> MGSDKIHHHHHHLPKLR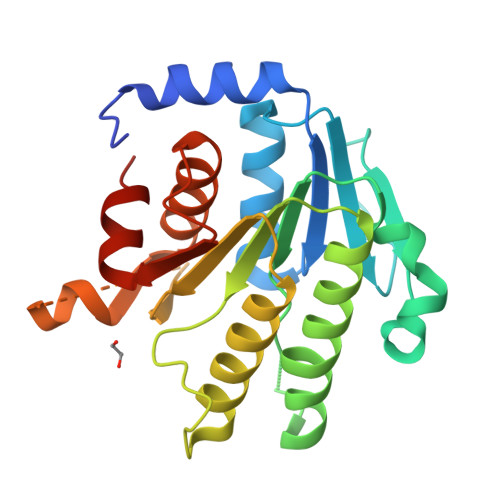EDFKMQNKSVFILGASGETGKVLLKEILGQNLFSKVTLIGRRKLTFEEEAYKNVNQEVVDFEKLDVYASAFQGHDVGFCCLGTTRSKAGAEGFVRVDRDYVLKSAELAKAGGCKHFNLLSSRGADKSSSFLYLQVKGEVEAKVEELKFDRLSVFRPGVLLCDRQESRPGEWLARKFFGSLPDSWASGYAVPVVTVVRAMLNNLVSPSSGQMELLENKAILHLGKDRDVPKL> MNLPTAQEVQGLMARFIELVDVGDIEAIVQMYADDATVENPFGQPPIHGREQIAAF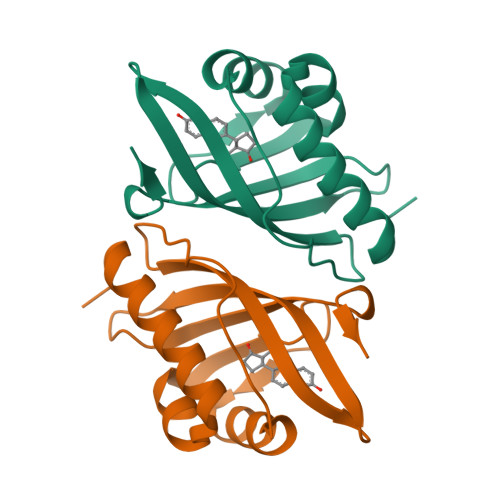YRQGLGGGKVRACLTGPVRASHNGCGAMPFRVEMVWNGQPCALDVIDVMRFDEHGRIQTMQAYWSEVNLSVREPQ> SMPRFVVQEHHARRLHWDLRLEMDNVLKSWALPKGVPEKRGVKRLAIETEDHDLSYIDFEGRIPEGMYGAGEVKIWDSGEYELLERTENKI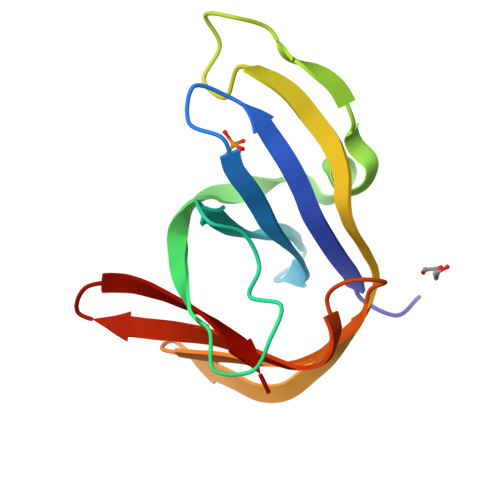KFLAKGRKMNGEYVLIKTKVGWLLMKA N-methyl-N-[(1S,3r)-3-methyl-3-{[(6M,8S)-6-(1-methyl-1H-pyrazol-4-yl)pyrazolo[1,5-a]pyrazin-4-yl]oxy}cyclobutyl]propanamide 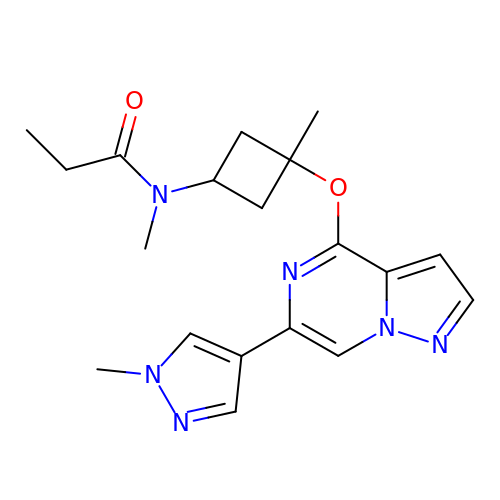| C19 H24 N6 O2 | MOIIQKULMWBCCK-QUWSVYMGSA-N> APTTLPPCKGSYF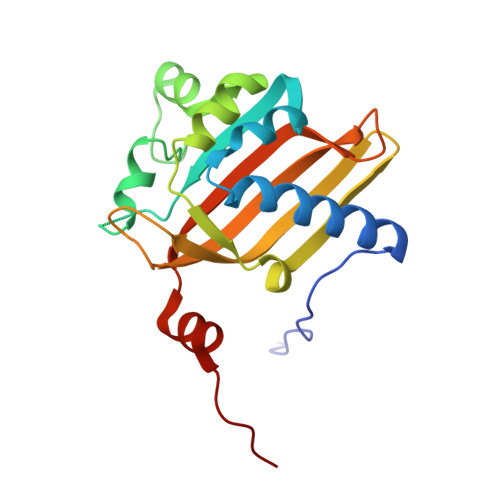GTENLKSLVLHFLQQYYAIYDSGDRQGLLDAYHDGACCSLSIPFIPQNPARSSLAEYFKDSRNVKKLKDPTLRFRLLKHTRLNVVAFLNELPKTQHDVNSFVVDISAQTSTLLCFSVNGVFKEVDGKSRDSLRAFTRTFIAVPASNSGLCIVNDELFVRNASSEEIQRAFAMPAPTP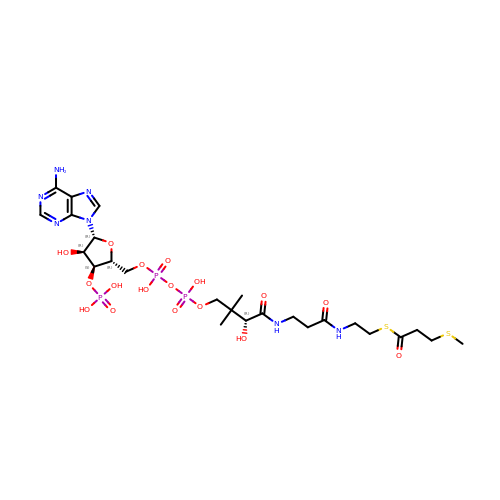3-methylmercaptopropionate-CoA (MMPA-CoA) | C25 H42 N7 O17 P3 S2 | SIEFLYWJLBNLAM-CITAKDKDSA-N>[2x]MMSETAPLPSASSALEDKA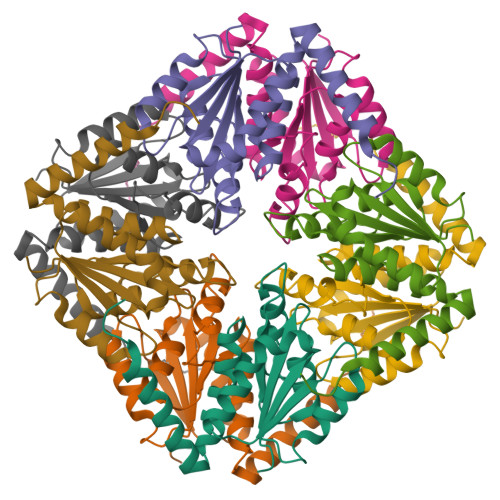ASAPVVGIIMGSQSDWETMRHADALLTELEIPHETLIVSAHRTPDRLADYARTAAERGLNVIIAGAGGAAFLPGMCAAWTRLPVLGVPVESRALKGMDSLLSIVQMPGGVPVGTLAIGASGAKNAALLAASILALYNPALAARLETWRALQTASVPNSPITEDK> GESWQKRYDSLQKIVEKQQQKMDQLRSQVQSLEQEVAQEEGTSQALREEAQRRDSALQQLRT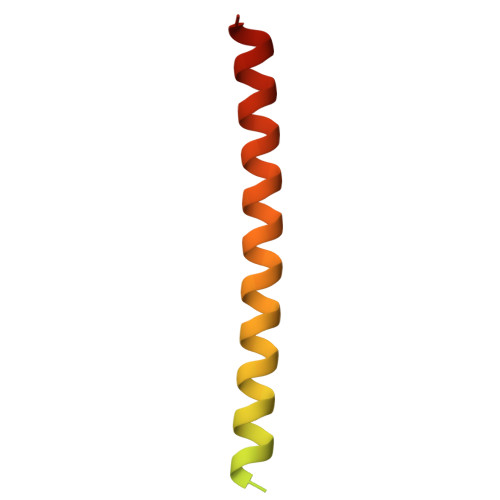AVKELSVQNQDLIEKNLTLQEHLRQA Thioredoxins (TRX) are small globular proteins of about 100–110 residues, which are conserved in all living organisms. They participate in multiple critical redox-reactions via the reversible oxidation of the active site CXXC catalytic motif1. Two TRX forms were described in Escherichia coli, Trx1 and Trx22. The former, called EcTRX throughout this work, is a widely used experimental model for investigating the molecular basis of protein stability, folding and function.

Despite being monomeric in solution, non-crystallographic symmetry is observed for the E101G and N106A mutants (two molecules per ASU) and for the L107A variant (seven molecules per ASU). Very weak electron density was observed for one of the L107A monomers, which was mostly modeled based on non-crystallographic symmetry restraints. No structural perturbations are found near the mutation site for the E101G and L107A mutants, which illustrate the robustness of the CTH element to sequence changes. The local effect involving loops centered in residues 20 and 83, as already mentioned, is observed for the L107A mutant and, in a lesser extension, for the E101G variant. Regarding cavities of the L107A mutant, the outcome of this substitution is a slight increase in the solvent-exposed surface, as Leu107 is a partially exposed residue. The four EcTRX mutants were crystallized in the oxidized form, and numerous protein-metal interactions were observed as a result of the Cu(II)-salt added for crystallization, as it was previously observed for the wild-type variant. Notably, the four variants crystallized in different crystal systems, comprising monoclinic, triclinic, orthorhombic and trigonal space groups, for L94A, E101G, N106A and L107A respectively. As expected from solution experiments, the global structures of the four variants are mainly unchanged compared to wild-type EcTRX, with main-chain root-mean-square deviation of atomic position (RMSD) differences of 0.59, 0.48, 0.62 and 0.48 Å for L94A, E101G, N106A and L107A, respectively. We found that global stability of the variants is progressively altered from 8.1 (wild-type), 7.8 (N106A), 7.4 (L94A), 7.2 (E101G) to 5.8 kcal mol−1 (L107A). For the L107A structure, B-factors were treated using TLS refinement, with one TLS group per protein chain. For variant L107A, the drop was a 2:1 mix of protein (10 mg/ml) and reservoir solution (100 mM sodium acetate, 4 mM CuSO4, 18% ethanol, pH 4.25).

>MSDKIIHLTDDSFDTDVLKADGAILVDFWAEWCGPCKMIAPILDEIADEYQGKLTVAKLNIDQNPGTAPKYGIRGIPTLLLFKNGEVAATKVGALSKGQLKEFLDANAA[7x]> SAWRKAGISYAAYLNVAAQAIRSSLKTELQTASVLNRSQTD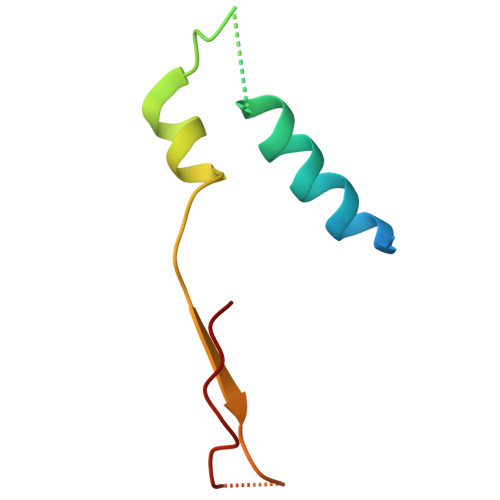AFYTQYKNGTAASEPTPITK>QVVSQGWKYFKGNFYYFSLIPKTWYSAEQFCVSRNSHLTSVTSESEQEFLYKTAGGLIYWIGLTKAGM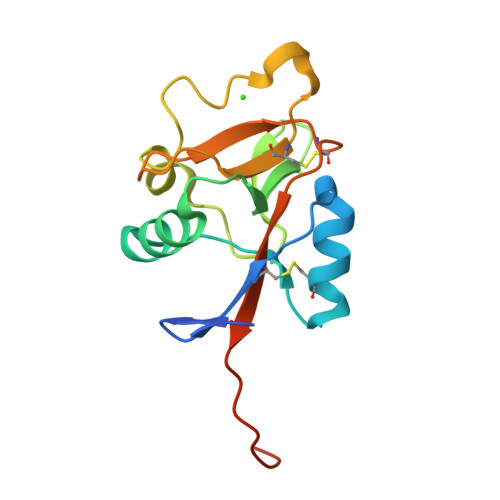EGDWSWVDDTPFNKVQSVRFWIPGEPNNAGNNEHCGNIKAPSLQAWNDAPCDKTFLFICKRPYVPSEPSAWSHPQFEK[4x]> H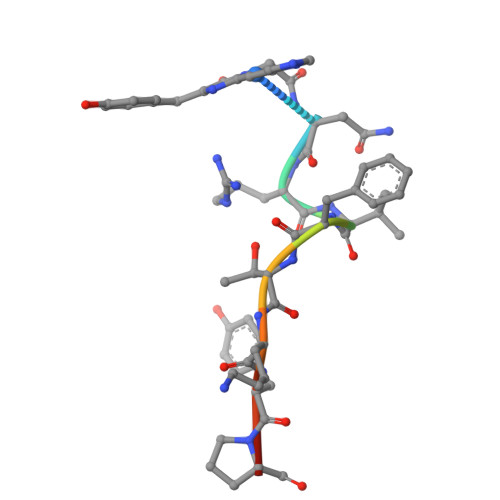YGNRVFTKYPR> DIAALLI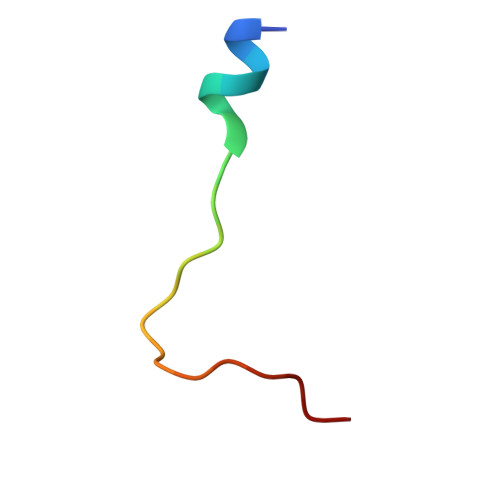AAGADVNAHAKGAFF> MAHVVILGAGTGGMPAAYEMKEALGSGHEVTLISANDYFQFVPSNPWVGVGWKERDDIAFPIRHYVERKGIHFIAQSAEQIDAEAQNITLADGNTVHYDYLMIATGPKLAFENVPGSDPHEGPVQSICTVDHAERAFAEYQALLREPGPIVIGAMAGASAFGPAYEYAMIVASDLKKRGMRDKIPSFTFITSEPYIGHLGIQGVGDSKGILTKGLKEEGIEAYTNCKVTKVEDNKMYVTQVDEKGETIKEMVLPVKFGMMIPAFKGVPAVAGVEGLCNPGGFVLVDEHQRSKKYANIFAAGIAIAIPPVETTPVPTGAPKTGYMIESMVSAAVHNIKADLEGRKGEQTMGTWNAVCFADMGDRGAAFIALPQLKPRKVDVFAYGRWVHLAKVAFEKYFIRKMKMGVSEPFYEKVLF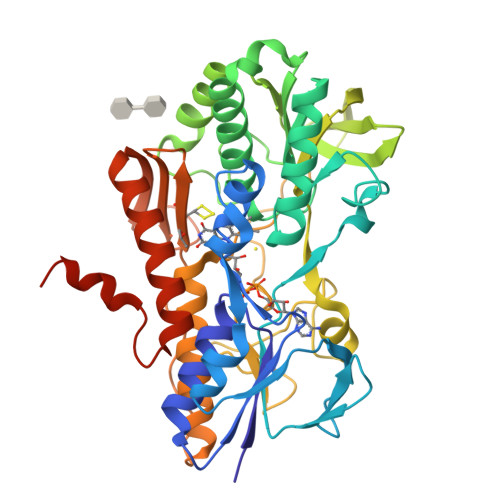KMMGITRLKEEDTHRKAS> 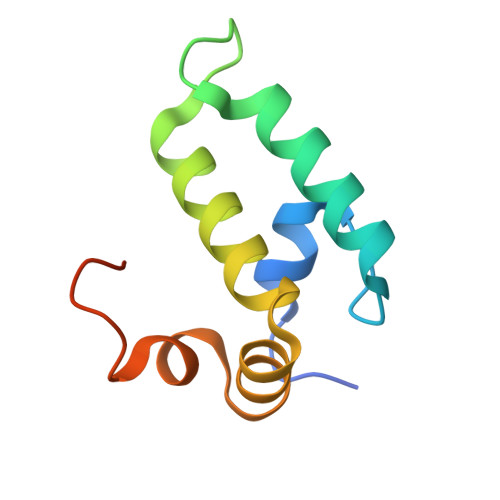SNAMVKETKLYDLLGVSPSANEQELKKGYRKAALKYHPDKPTGDTEKFKEISEAFEILNDPQKREIYDQYGLEAARSGGPSFGPGGPGGAGG> AFPISDITVVSERTDASTAYLSDWFVVSFVFSTAGSDETIAGDATIEVSIPNELEFVQYPDSVDPSVSEFFTTAGVQVLSTAFDYDSHVLTFTFSDPGQVITDLEGVVFFTLKLSEQFTESASPGQHTFDFETSDQTYSPSVDLVALDRSQPIKLSNAVTGGVEWFVDIPGAFGDITN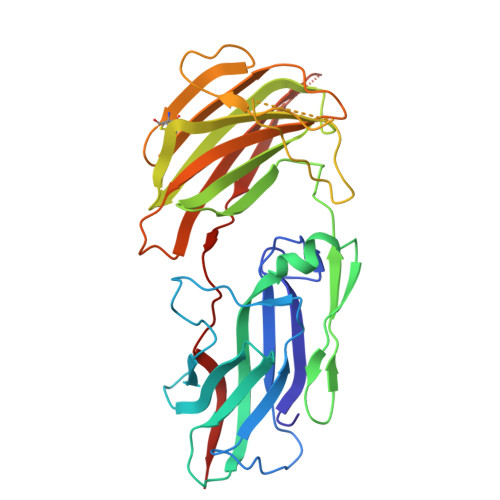IDISTVQTPGTFDCSEVKYAVGSSLNEFGDFTPQDRTTFFSNSSSGEWIPITPASGLPVESFECGDGTISLSFAGELADDEVLRVSFLSNLADDVLEVQNVVNVDLTTADSRKRALTSFVLDEPFYRASRTDTAAFEAFAAV> MSRSKRDNNFYSVEIGDSTFTVLKRYQNLKPIGSGAQGIVCAAYDAILERNVAIKKLSRPFQNQTHAKRAYRELVLMKCVNHKNIIGLLNVFTPQKSLEEFQDVYIVMELMDANLCQVIQMELDHERMSYLLYQML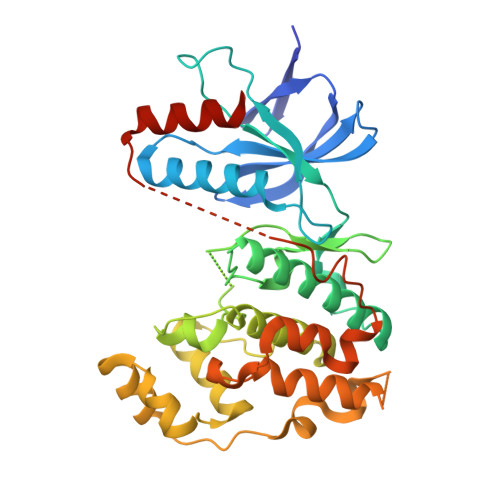CGIKHLHSAGIIHRDLKPSNIVVKSDCTLKILDFGLARTAGTSFMMTPYVVTRYYRAPEVILGMGYKENVDIWSVGCIMGEMIKGGVLFPGTDHIDQWNKVIEQLGTPCPEFMKKLQPTVRTYVENRPKYAGYSFEKLFPDVLFPADSEHNKLKASQARDLLSKMLVIDASKRISVDEALQHPYINVWYDPSEAEAPPPKIPDKQLDEREHTIEEWKELIYKEVMDLHHHHHH> IKELKMSKDEIKREYKEMEGSPEIKSKRRQFHQEIQSRNMRENVKRSSVVVAAATHIAIGILYKRGETPLPLVTFKYTDAQVQTVRKIAEEEGVPILQRIPLARALYWDALVDHYIP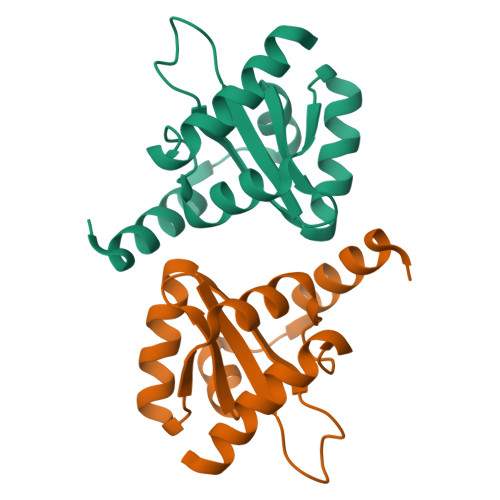AEQIEATAEVLRWLERQNIEKQHSEML>GIDPFTSKDTGKVGEKSAEISAKDTLGKAVKLADDNTSLKVLVFFQNGCPSCLKELPSLDEFIQNHPNKISVYAINSIDNANVVKVLAEQFDFKNVKVLKDDLKITNDRYAVFATPTTIIIKDG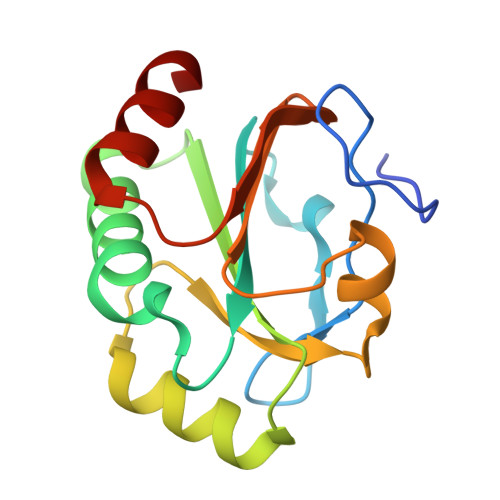MIKDRILGEKPWEFFESKLISLL[2x]>MAPKSSSSGSKKKSSASSNSADAKASKFKLPAEFITRPHPSKDHGKETCTAYIHPNVLSSLEINPGSFCTVGKIGENGILVIARAGDEEVHPVNVITLSTTIRSVGNLILGDRLELKKAQVQPPYATKVTVGSLQGYNILECMEEKVIQKLLDDSGVIMPGMIFQNLKTKAGDESIDVVITDASDDSLPDVSQLDLNMDDMYGGLDNLFYLSPPFIFRKGSTHITFSKETQANRKYNLPEPLSYAAVGGLDKEIESLKSAIEIPLHQPTLFSSFGVSPPRGILLHGPPGTGKTMLLRVVANTSNAHVLTINGPSIVSKYLGETEAALRDIFNEARKYQPSIIFIDEIDSIAPNRANDDSGEVESRVVATLLTLMDGMGAAGKVVVIAATNRPNSVDPALRRPGRFDQEVEIGIPDVDARFDILTKQFSRMSSDRHVLDSEAIKYIASKTHGYVGADLTALCRESVMKTIQRGLGTDANIDKFSLKVTLKDVESAMVDIRPSAMREIFLEMPKVYWSDIGGQEELKTKMKEMIQLPLEASETFARLGISAPKGVLLYGPPGCSKTLTAKALATESGINFLAVKGPEIFNKYVGESERAIREIFRKARSAAPSIIFFDEIDALSPDRD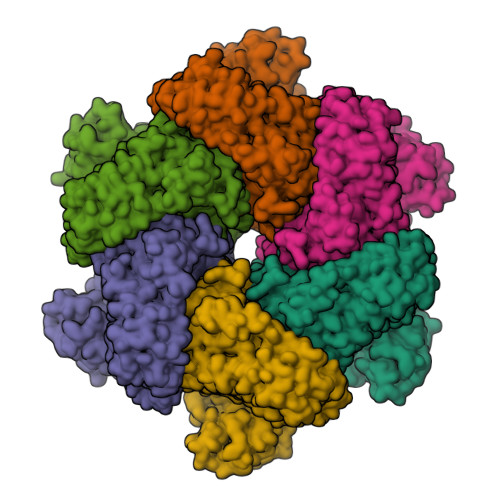GSSTSAANHVLTSLLNEIDGVEELKGVVIVAATNRPDEIDAALLRPGRLDRHIYVGPPDVNARLEILKKCTKKFNTEESGVDLHELADRTEGYSGAEVVLLCQEAGLAAIMEDLDVAKVELRHFEKAFKGIARGITPEMLSYYEEFALRSGSSS[6x]(2E)-2-cyano-3-[3-(1H-pyrazol-4-yl)phenyl]prop-2-enamide | C13 H10 N4 O | 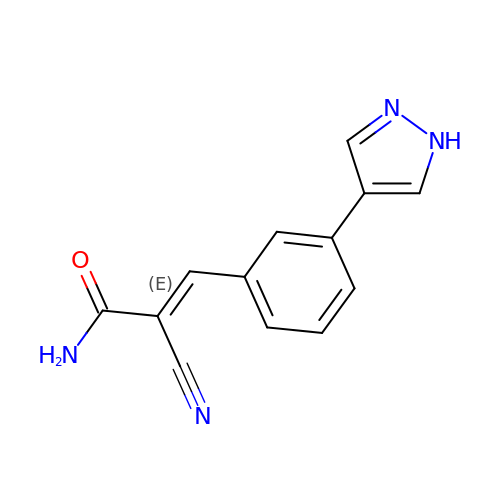YCZXMEXRJXFIIS-VZUCSPMQSA-N> GSHMRTPIIAGNWKMHYTIDEAVKLVEELKPLVKDAKCEVVVCPTFVCLDAVKKAVEGTNIKVGAQNMHFEEKGAFTGEIAPRMLEAMNIDYVIIGHSERREYFNE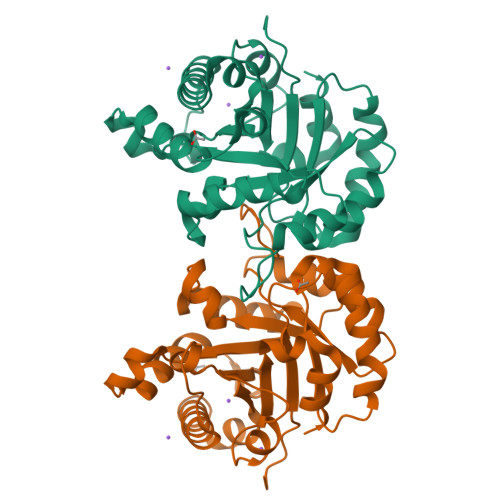TDETCNKKVKAAFAHNLTPILCCGETLEQRENGTTNDVIKAQITADLEGLTKEQAEKVVIAYEPIWAIGTGKTATSDQANETIAAIRAMVAEMFGQEVADKVRIQYGGSVKPNTIAEQMAKSDIDGALVGGASLVAADFAQIVNY>MGGSSHHHHHHSSGLVPRGSGGLTHRKFGGSGGSPFSGLSSIAVRSGSFLDAIIIDGVHHGGSGGNLSPTFTFGSGEYISNMTIRSGDFIDNISFETNMGRRFGPYGGSGGSANTLSNVKVIQINGSAGDFLDSLDIYYE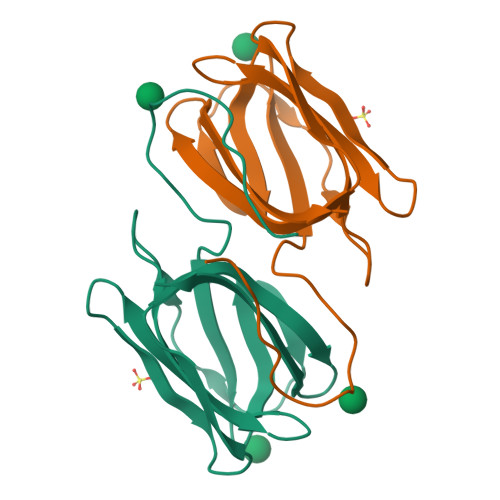QY[3x]>[2x]SMSLLDAHIPQLIASEANFGAKAALMRSTIAQAEQAAMSSQAFHMGEASAAFQAAHARFVEVSAKVNALLDIAQLNIGDAASSYVAQDAAAASTYTGI;>MSQIMYNYPAMLAHAAEMNTYSGALHAVGADIAAEQHALASAWQGDTGMTYQAWQAQWNQAMEELVRAYRAMATTHEQNTMAMSARDQAEGAKWGTHHHHHH[2x]

Of particular interest are the Esx complexes which are dimers of two subunits (ESAT-6, early secreted antigen of 6 kDa; and CFP-10, culture filtrate protein of 10 kDa) and which are secreted across the cytoplasmic membrane by Type VII secretion (T7S) systems. Mycobacterial ESX secretion systems have been shown to be involved in a variety of physiological processes including conjugation in a non-pathogenic mycobacterium, iron and/or zinc acquisition by both pathogenic and non-pathogenic mycobacterial species, and virulence of pathogenic mycobacteria. The overall architecture of the complexes is similar to known Esx structures in that each heterodimer forms a four helix bundle with the CFP-10 and ESAT-6 subunit homologs each contributing an α-helical hairpin to the complex. The subunit interfaces in the four-helix bundles of the Esx complexes are similar to those of the previously determined Esx complex structures in that the intermolecular interface between the CFP-10 and ESAT-6 subunits is largely hydrophobic.

Using this expression approach we expressed and purified six Esx complexes and determined the crystal structures of M. abscessus EsxEF (EsxEFma), encoded by the MAB_3112 and MAB_3113 genes, M. smegmatis EsxGH (EsxGHms), encoded by the MSMEG_0620 and MSMEG_0621 genes, and M. tuberculosis EsxOP (EsxOPmt), encoded by the Rv2346c and Rv2347c genes, at resolutions of 1.96 Å, 2.70 Å, and 2.55 Å, respectively. The structures of these complexes were determined by single wavelength anomalous diffraction (EsxEFma and EsxGHms) and multiple wavelength anomalous diffraction (EsxOPmt) at resolutions of 3.0 Å, 2.70 Å, and 2.55 Å, respectively. The α-helices of each subunit are connected by a flexible loop containing the canonical ESAT-6/CFP-10 signature motif (Trp-Xaa-Gly; WXG) although the EsxGms CFP-10 homolog contains a modified motif (His-Xaa-Gly). The WXG-containing loops are well ordered in the EsxGHms complexes and in most of the EsxEFma complexes but the majority of the connecting loops are disordered in the EsxOPmt subunit structures. The average amount of buried surface area in the subunit interfaces varies considerably [EsxEFma, ∼1605 Å2; EsxGHms, ∼1555 Å2; EsxOPmt (form I), ∼1025 Å2; and EsxOPmt (form II), ∼1175 Å2] and the percentage of the surface of each subunit buried in the complex interface is also highly variable, from 13.5–33%, and is related to the degree to which the termini of the subunits are ordered and to the conformations that they adopt. The C-termini of the CFP-10 homolog subunits of our EsxGHms and EsxOPmt (forms I and II) structures, which contain the secretion motif, are ordered and adopt helical structures; in the EsxOPmt structure the secretion motif containing helix is an extension of the C-terminal helix of the α-helical hairpin while in EsxGHms the secretion motif is primarily contained in a short, 13 amino acid, helix linked to the α-helical hairpin by a short turn.>GSHMGGIEVLDVKTGPDSTTTIEAYLNPRVGQNWGFSTEITVASNGYNDAPHLTEIPCYSSARISLPLLNEDITSPTLLMWEAVSVKTEVVGISSMLNMHSYGLRAFGGYGGGYTIEGSHIHFFSVGGEPLDLQGLMQNHSTQYPSPLVGPKKPDGTTDDSAQVLNPIYKAKLDKDATYPIECWCPDPSRNENSRYFGSYTGGVETPPVLSFTNTSTTILLDENGVGPLCKGDGLYLSSADVAGTFVQQTSQKQYWRGLPRYFNITLRKRAVKN[40x]

Polyomaviruses are small double-stranded DNA (dsDNA) viruses with a circular genome of approximately 5,000 bp. All glycan-binding polyomaviruses analyzed to date engage oligosaccharide (glycan) structures featuring terminal sialic acids that in mammals are usually presented either on gangliosides, which are molecules composed of a glycosphingolipid, i.e., a ceramide and an oligosaccharide, or on glycoproteins, which contain mostly complex and branched oligosaccharides attached to amino acids during co- and posttranslational modification steps. These sialylated glycan structures interact with loop regions at the outer margin of the major capsid protein VP1, at the apical surface of the polyomavirus capsid, as revealed by X-ray crystallography and cryoelectron microscopy. The VP1 surface exhibits an astonishing plasticity, providing virus-specific interactions for a range of Neu5Ac linkage types and further specific characteristics of Neu5Ac-containing glycans.

In order to define the ligand binding properties of the three animal viruses ShPyV, GhPyV, and FiPyV, we conducted crystal soaking experiments with sialylated glycans, which yielded additional electron density for the glycan ligand so that we could solve and refine complex structures for ShPyV VP1 with 6′SLN and 3′SLN, GhPyV VP1 with 2-O-Me-Neu5Ac, and FiPyV VP1 with 2-O-Me-Neu5Ac to 1.6 Å, 1.65 Å, 1.95 Å, and 2.8 Å resolution, respectively. FiPyV VP1, which was also derivatized with 2-O-Me-Neu5Ac, forms interactions with Neu5Ac that are very similar to those observed in GhPyV and ShPyV VP1. The methyl group of the N-acetyl moiety reaches into a shallow groove formed by residues T58, V59, A60, D66, A67, P68, E72, and H117ccw. The N-acetyl amide is recognized by the hydroxyl group of T58. The R122ccw side chain interacts with the Neu5Ac glycerol moiety, contacting the hydroxyl groups of C-8 or C-9, depending on the VP1 chain. Residue H69 of the FiPyV VP1 contacts both the Neu5Ac carboxylate group and the E72 side chain, thereby providing for an additional hydrogen bond between the protein and the putative Neu5Ac-containing receptor. However, FiPyV did not hemagglutinate chicken or human erythrocytes, suggesting an alternative receptor specificity compared to that of the related viruses, likely influenced by residues surrounding the conserved BC2 loop Neu5Ac-binding site.> MLCRTFLRQFRMSGGDMFVEYKVLSRDHRRSIRVEDAIVDPTFKRTVLPLGWLELLRSPSLRLPTGYFVEETVHVSLPNATSNGGKKEARPQKGGFASGSPSVGRNEANAIIAGPVVLYITGQSVPVVLNPYFVPEGTWDMRTRDGELDLRL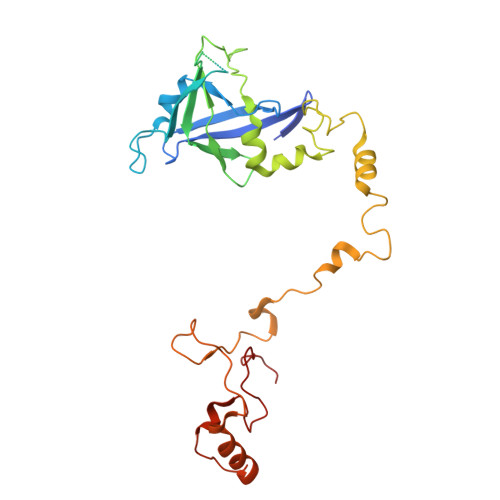GMDAIEQCTLFSELRPGGLLYGKLPENPNVRRNESLRATLGRYGMKCDLAESPLVPRPWTRMRYMFIDELQRGPKLTEFVGHNPRNGTPWRFSQNTKYFRIGIWRDTIRRNDMNEGLHAHSSWQKSPQQSVPEVRFLAPYP>MDYKDDDDKMPSPTTVPVATAGRLAEPYIDPAAQVHAIASIIGDVRIAAGVRVAAGVSIRADEGAPFQVGKESILQEGAVIHGLEYGRVLGDDQADYSVWIGQRVAITHKALIHGPAYLGDDCFVGFRSTVFNARVGAGSVIMMHALVQDVEIPPGRYVPSGAIITTQQQADRLPEVRPEDREFARHIIGSPPVIVRSTPAATADFHSTPTPSPLRPS[2x];>[4x]FQSNMHLPPLEPPISDRYFASGEVTIAADVVIAPGVLLIAEADSR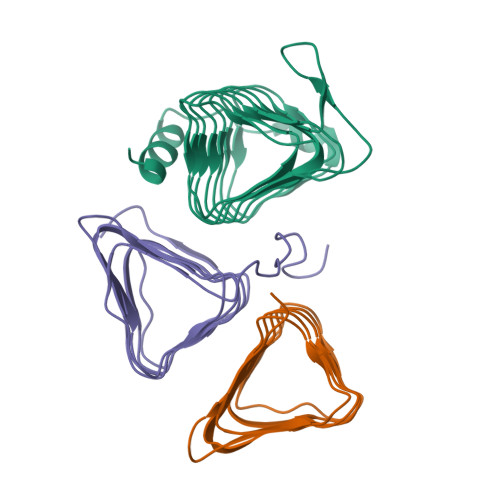IEIASGVCIGLGSVIHARGGAIIIQAGALLAAGVLIVGQSIVGRQACLGASTTLVNTSIEAGGVTAPGSLLSAETPP>YEQDKTYKITVLHTNDHHGHFWRNEYGEYGLAAQKTLVDGIRKEVAAEGGSVLLLSGGDINTGVPESDLQDAEPDFRGMNLVGYDAMAIGNHEFDNPLTVLRQQEKWAKFPLLSANIYQKSTGERLFKPWALFKRQDLKIAVIGLTTDDTAKIGNPEYFTDIEFRKPADEAKLVIQELQQTEKPDIIIAATHMGHYDNGEHGSNAPGDVEMARALPAGSLAMIVGGHSQDPVCMAAENKKQVDYVPGTPCKPDQQNGIWIVQAHEWGKYVGRADFEFRNGEMKMVNYQLIPVNLKKKVTWEDGKSERVLYTPEIAENQQMISLLSPFQNKGKAQLEVKIGETNGRLEGDRDKVRFVQTNMGRLILAAQMDRTGADFAVMSGGGIRDSIEAGDISYKNVLKVQPFGNVVVYADMTGKEVIDYLTAVAQMKPDSGAYPQFANVSFVAKDGKLNDLKIKGEPVDPAKTYRMATLNFN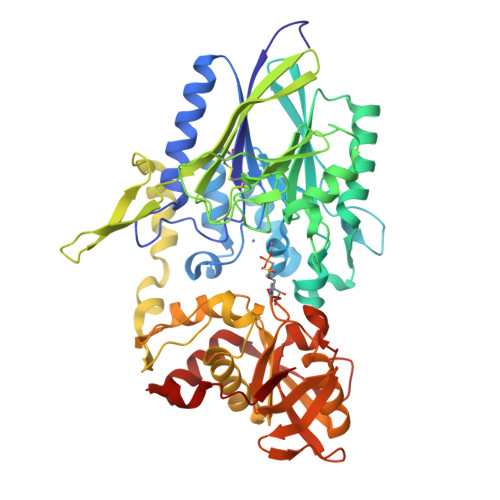ATGGDGYPRLDNKPGYVNTGFIDAEVLKAYIQKSSPLDVSVYEPKGEVSWQ[4x]> VFHKIRNEDLIFNESLGQGTFTKIFKGVRREVGDYGQLHETEVLLKVLDKAHRNYSES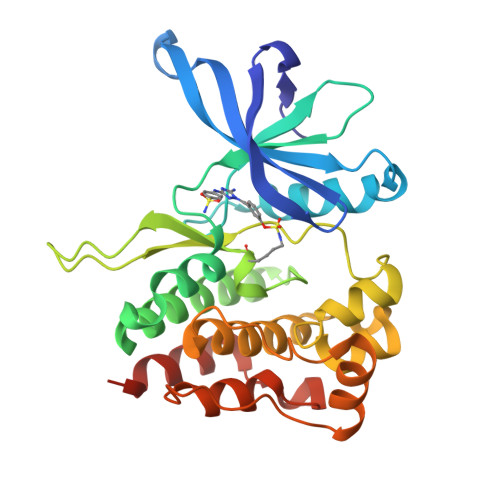FFEAASMMSKLSHKHLVLNYGVCVCGDENILVQEFVKFGSLDTYLKKNKNCINILWKLEVAKQLAWAMHFLEENTLIHGNVCAKNILLIREEDRKTGNPPFIKLSDPGISITVLPKDILQERIPWVPPECIENPKNLNLATDKWSFGTTLWEICSGGDKPLSALDSQRKLQFYEDRHQLPAPKWAELANLINNCMDYEPDHRPSFRAIIRDLNSLFHHHHHH> MATQHPIGKKTACVVGGTGFVASLLVKLLLQKGYAVNTTVRDPDNQKKVSHLLELQELGDLKIFRADLTDELSFEAPIAGCDFVFHVATPVHFASEDPENDMIKPAIQGVVNVMKACTRAKSVKRVILTSSAAAVTINQLDGTGLVVDEKNWTDIEF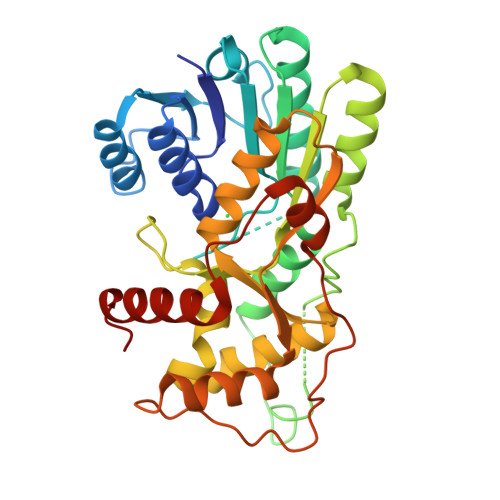LTSAKPPTWGYPASKTLAEKAAWKFAEENNIDLITVIPTLMAGSSLTSDVPSSIGLAMSLITGNEFLINGMKGMQMLSGSVSIAHVEDVCRAHIFVAEKESASGRYICCAANTSVPELAKFLSKRYPQYKVPTDFGDFPPKSKLIISSEKLVKEGFSFKYGIEEIYDESVEYFKAKGLLQN> FMP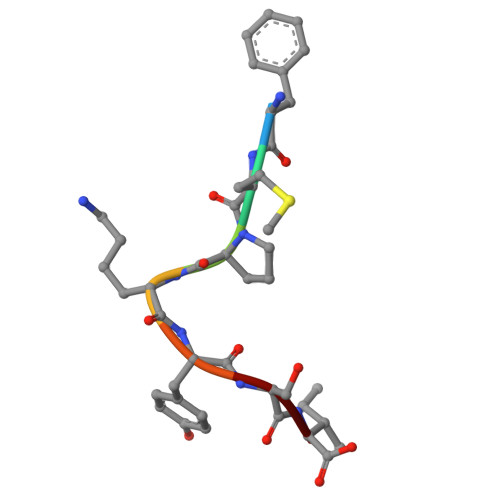KYSI>[2x]IE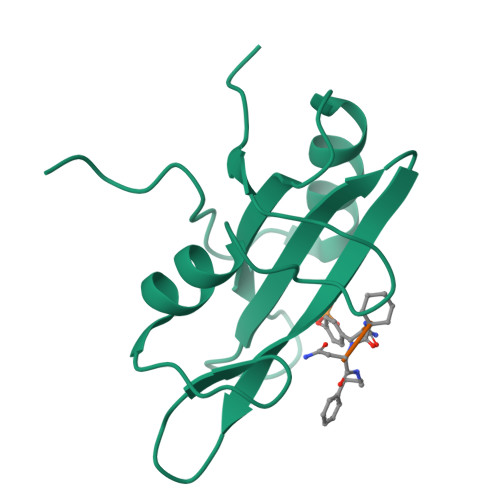MKPHPWFFGKIPRAKAEEMLSKQRHDGAFLIRESESAPGDFSLSVKFGNDVQHFKVLRDGAGKYFLWVVKFNSLNELVDYHRSTSVSRNQQIFLRDIEQVPQQPTYVQAHHHHHH>[4x]GMACGLVASNLNLKPGECLRVRGEVAPDAKSFVLNLGKDSNNLCLHFNPRFNAHGD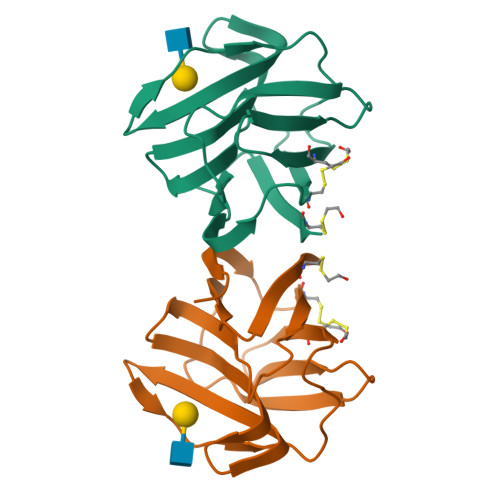ANTIVCNSKDGGAWGTEQREAVFPFQPGSVAEVCITFDQANLTVKLPDGYEFKFPNRLNLEAINYMAADGDFKIKCVAFD Glutaredoxins (GRXs) are thioredoxin superfamily members exhibiting thiol-disulfide oxidoreductase activity and/or iron-sulfur (Fe-S) cluster binding capacities. CrGRX2 is a class I GRX member that possesses a classical YCPYC signature with two cysteine residues present at positions 27 and 30, whereas a third, non-conserved, cysteine is present at position 56. In conclusion, using the roGFP2 as a model protein substrate, we showed that CrGRX2 catalyzes both protein glutathionylation and deglutathionylation reactions in the presence of GSSG and GSH, respectively. In addition, this work demonstrates that C. reinhardtii GRX2 has the capacity to bind a [2Fe–2S] cluster despite having the canonical CPYC active site signature that was shown to prevent Fe–S cluster binding in some other GRXs.

The crystal structure of CrGRX2 was solved at a high-resolution using synchrotron radiation (1.5 Å, CrGRX2red) while a lower resolution was obtained using a laboratory source (2.4 Å, CrGRX2SS). Both crystals were isomorphous and the structures were highly similar (root-mean-square deviation (r.m.s.d.) of 0.10 Å for the superimposition of 107 pairs of Cα atoms). Only one difference was noted: Cys27 and Cys30 form a disulfide bond in the CrGRX2SS structure while they were reduced in CrGRX2red. The equivalent distance of 3.2 Å in the CrGRX2red structure indicates that the disulfide bond was most likely broken during the synchrotron data collection. CrGRX2 crystallized in space group P3221 with a single molecule of CrGRX2 (Met1-Leu107 residues) per asymmetric unit. The overall fold of CrGRX2 showed four mixed β-strands in a central core structure surrounded by five α-helices. The four-stranded β-sheet is sandwiched by α-helices α1 and α3 on one side and α-helices α2, α4, and α5 on the other side. We found an acetate molecule originating from the crystallization medium at the position usually occupied by the carboxylic acid group of the γ-glutamyl moiety of GSH. The amine groups of Gly85 and Asp86, located just after two conserved glycine residues forming a structural kink, help stabilizing the acetate ion through hydrogen bonding.

> MGKAEAINEIQKAVASNKVIVYSKTYCPYCVKAKNALNQFIAGKYTVVELENRADCDAMQDALLDITGGRSVPRVFINGKFLGGGDDTAAAASNGTLEKLLQEAGAL>[5x]MSDIFNSPQNKASILTALMKSTTGDVEDVLIPKRFRPAKDPLDSPQAAAQFLKDNKYRILRPRAIPTMVELETDAALPRLRQMVEDGKLKDTVSVPEGTTAFYPKYYPFHKPDHDEVGTFGAPDITLLKQLTFFLLENDFPTGPETLRQVREAIATLQYGSGSYSGQLNRLLAMKGVATGRNPNKTPKTVGYTNEQLAKLLEQTLPINTPKHEDPDLRWAPSWLINYTGDLSTDKSYLPHVTIKSSAGLPYIGKTKGDTTAEALVLADSFIRDLGRAATSADPEAGVKKTITDFWYLSCGLLFPKGERYTQVDWDKKTRNIWSAPYPTHLLLSMVSTPVMNESKLNITNTQTPSLYGFSPFHGGMDRIMTIIRDSLDNDEDLVMIYADNIYILQDNTWYSIDLEKGEANCTPQHMQAMMYYLLTRGWTNEDGSPRYNPTWATFAMNVAPSMVVDSSCLLMNLQLKTYGQGSGNAFTFLNNHLMSTIVVAEWVKAGKPNPMTKEFMDLEEKTGINFKIERELKNLRETIVEAVETAPQDGYLADGSDLPPIRPGKAVELDLLGWSAIYSRQMEMFVPVLENERLIASAAYPKGLENKALARKPGAEIAYQIVRYEAIRLVGGWNNPLLETAAKHMSLDKRKRLEVKGIDVTGFLDDWNNMSEFGGDLEGITLSEPLTNQTLVDINTPLDSFDPKARPQTPRSPKKTLDEVTTAITSGTYKDPKSAVWRLLDQRTKLRVSTLRDQALALKPASSSVDNWAEATEELAQQQQLLMKANNLLKSSLTETREALEKTGHHHHHH

Members of the family Birnaviridae possess bi-segmented double-stranded RNA (dsRNA) genomes and form virions with non-enveloped single-shelled icosahedral capsids. From sequence analysis it was proposed that the RdRPs of Birnaviridae possess a non-canonical active site where the polymerase sequence motifs are re-ordered C-A-B, motif C containing ADN in place of the conserved GDD catalytic residues. An additional unusual feature of birnavirus RdRPs is their ability to self-guanylylate: auto-catalyzing the covalent addition of a GMP moiety to a serine residue of the polymerase in a template-independent manner to form VP1pG. We have cloned, expressed and solved the structure of the RdRP VP1 from IPNV in both its apo form and bound to a catalytic metal (magnesium).

A second construct lacking the C-terminal 55 residues (ΔC55) was therefore cloned, expressed, purified and crystallised. These crystals diffracted well and the structure was solved by molecular replacement using the structure of IBDV VP1 as a search model. The IPNV polymerase closely resembles IBDV VP1, with an r.m.s. deviation in Cα positions of 1.2 Å over 678 residues. The structure of IPNV VP1 confirms the previously-identified rearrangement of the catalytic palm domain, with the non-canonical ADN catalytic motif (residues 387–389) lying at the apex of a β-hairpin in the active site. Strong electron density was observed near the outer edge of the palm domain, between the side chains of N184, N409 and N514 and the backbone carbonyl oxygen atoms of V177, N182 and G512. This feature, some 15 Å from the putative active site, was modeled as a K+ ion based on the strength of the electron density, the ligand-to-K+ distances of 2.6–2.8 Å and the hard nature of the six ligands. Additional electron density resembling a protein helix was observed in the active site cleft of both apo and Mg-bound ΔC55 VP1. Based on the presence of strong density suggesting a sulfur-containing methionine side chain, this helix was tentatively assigned as residues 11–19 from the otherwise-disordered N-terminal tail of the protein. As the 48 Å separating the final residue of the helix (M19) and the first residue of the polymerase domain (I31) is too great to be spanned by the intervening 10 residues, the N-terminal helix presumably derives from an adjacent polymerase domain in the crystal.> MKTVEIIEGIASG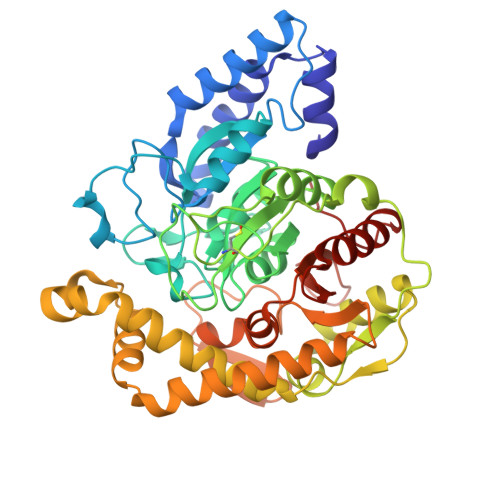RTSARDVCEEALATIGATDGLINAFTCRTVERARAEADAIDVRRARGEVLPPLAGLPYAVKNLFDIEGVTTLAGSKINRTLPPARADAVLVQRLKAAGAVLLGGLNMDEFAYGFTTENTHYGPTRNPHDTGRIAGGSSGGSGAAIAAGQVPLSLGSDTNGSIRVPASLCGVWGLKPTFGRLSRRGTYPFVHSIDHLGPLADSVEGLALAYDAMQGPDPLDPGCSASRIQPSVPVLSQGIAGLRIGVLGGWFRDNAGPAARAAVDVAALTLGASEVVMWPDAEIGRAAAFVITASEGGCLHLDDLRIRPQDFEPLSVDRFISGVLQPVAWYLRAQRFRRVYRDKVNALFRDWDILIAPATPISAPAIGTEWIEVNGTRHPCRPAMGLLTQPVSFAGCPVVAAPTWPGENDGMPIGVQLIAAPWNESLCLRAGKVLQDTGIARLKC> RLYRADSRPPDEIKRSGGLMPRGHNEYFDRGTQMNINLYDHARGTQTGFVRYDDGYVSTSLSLRSAHLAGQSILSGYSTYYIYVIATAPNMFNVNDVLGVYSPHPYEQEVSALGGIPY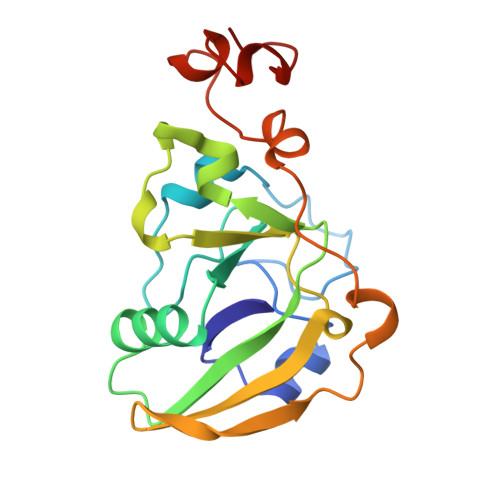SQIYGWYRVNFGVIDERLHRNREYRDRYYRNLNIAPAEDGYRLAGFPPDHQAWREEPWIHHAPQGCG>[2x]GAMGQTTFTELMQQLFLKLGLNHQVNENDVYTFEVDGHIQVLIACYHQQWVQLFS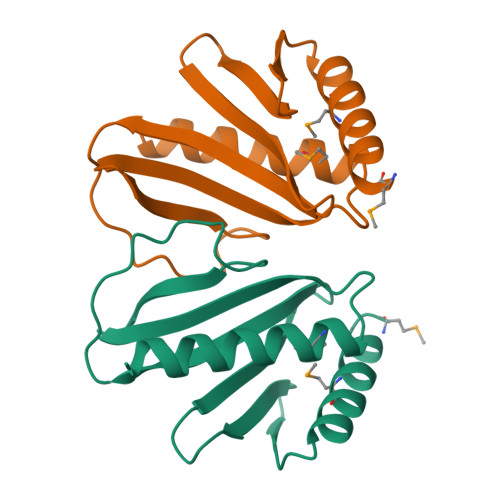ELGADLPTNDNLFGEHWPAHVQGRLDGKSILWSQQSLVGLDIDEMQAWLERFIDDIEQRKEPQNTKFQPN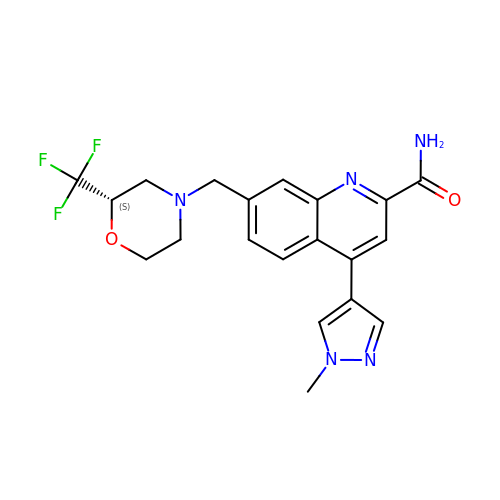4-(1-methylpyrazol-4-yl)-7-[[(2~{S})-2-(trifluoromethyl)morpholin-4-yl]methyl]quinoline-2-carboxamide | C20 H20 F3 N5 O2 | PUIAIYDBFPDZPF-SFHVURJKSA-N>GSSGSSGMQIGKIIKVSGPLVMAENMSEASIQDMCLVGDLGVIGEIIEMRQDVASIQVYEETSGIGPGEPVRSTGEALSVELGPGIISQMFDGIQRPLDTFMEVTQSNFLGRGVQLPALDHEKQWWFEATIEEGTEVSAGDIIGYVDETKIIQHKIMVPNGIKGTVQKIESGSFTIDDPICVIETEQGLKELTMMQKWPVRRGRPIKQKLNPDVPMIT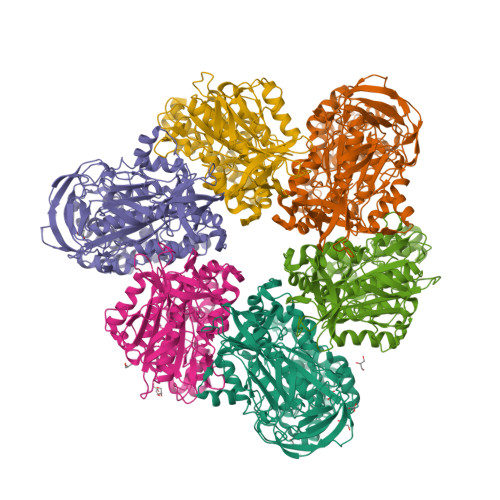GQRVIDTFFPVTKGGAAAVPGPFGAGKTVVQHQIAKWSDVDLVVYVGCGERGNEMTDVVNEFPELIDPNTGESLMERTVLIANTSNMPVAAREASIYTGITIAEYFRDMGYDVAIMADSTSRWAEALREMSGRLEEMPGDEGYPAYLGSRLAEYYERSGRVIALGSDQREGSITAISAVSPSGGDISEPVTQNTLRVVKVFWGLDSSLAQKRHFPSINWIQSYSLYSTEVGRYMDQILQQDWSDMVTEGMRILQEEEQLNEIVRLVGIDSLSDNDRLTLEVAKSIREDYLQQNAFDDVDTFTSREKQFNMLKVILTFGKEARKALSLGAYFNEIMEGTVAVRERISRSKYIPEEELAKISSINEEIKETIQLIVSE[6x];>[6x]GSSGSSGMIKEYRTIKEVVGPLMAVEKVSGVKYEELIEVRMQNGEIRRGQVLEVQEDKAMVQIFEGTSGINYKNSSVRFLGHPLQLGVSEDMIGRVFDGLGRPKDNGPEILPEKYLDINGEVINPIARDYPDEFIQTGISAIDHLNTLVRGQKLPVFSGSGLPHKELAAQIARQATVLDSSDDFAVVFAAIGITFEEAEFFMEDFRQTGAIDRSVMFMNLANDPAIERIATPRMALTAAEYLAYEKGMHVLVIMTDMTNYAEALREISAARREVPGRRGYPGYLYTNLATLFERAGRIRGLKGSVTQIPILTMPEDDKTHPIPDLTGYITEGQIILTRELYKSGIQPPIDVLPSLSRLKDKGTGAGKTREDHAATMNQLFAAYAQGKQAKELAVVLGESALSDIDKIYAKFAERFENEYVNQGFYTNRTITETLDLGWELLAMLPRTELKRIKDDLLDKYLP> MSESEAKSRSATPPSKAKQATPTTTAAANGEKKLTNKELKELKKQEKAAKRAAMKQANGISIEQQQQQAQMKKEKKQLQREQQQKREQKQKNANKKKQNERNVKKSTLFGHLETTEERRATILALTSAVSSPKTSRITAAGLMVPVVASALSGSNVLTASSLMPVGPNASSTVSASAPASTTTTLPASSAALSAGTSSASTNTPTAIQQEIASSNASDVAKTLASISLEAGEFNVIPGISSVIPTVLEQSFDNSSLISSVKELLLNKDLIHPSILLLTSHLAHYKIVGSIPRCIAMLEVFQIVIKDYQTPKGTTLSRNLTSYLSHQIDLLKKARPLSVTMGNAIRWLKQEISLIDPSTPDKAAKKDLCEKIGQFAKEKIELADQLIIDNASTQIEESTTIVTYGSSKVLTELLLHNAISLKKNIKVIVVDSRPLFEGRKMAETLRNAGVNVMYALITSLDTIFNMDVDYVFLGAHSILSNGFLY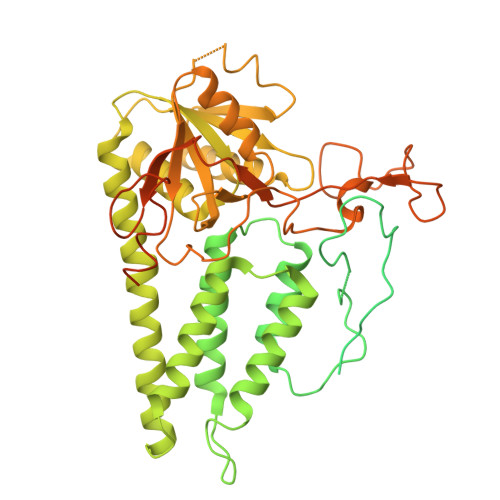SRAGTAMLAMSAKRRNIPVLVCCESLKFSQRVQLDSVTFNELADPNDLVNIDYENPVERRGNKGALLNQFIKERKFEKKKLAMENKPKGNKIGGKKGSEGESKDASNEEDSNSKNILDGWQELPSLNIVNILYDLTPPEYIKKVITEFGALPPSSVPVILREYKGSA>[4x]GMFASLIKRFQFVSVLDSNPQTKVMSLLGTIDNKDAIITAEKTHFLFDETVR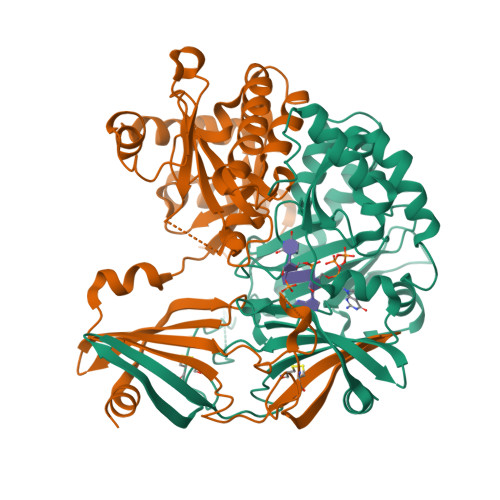RPSQDGRSTPVLYNCENEYSCINGIQELKEITSNDIYYWGLSVIKQDMESNPTAKLNLIWPATPIHIKKYEQQNFHLVRETPEMYKRIVQPYIEEMCNNGRLKWVNNILYEGAESERVVYKDFSEENKDDGFLILPDMKWDGMNLDSLYLVAIVYRTDIKTIRDLRYSDRQWLINLNNKIRSIVPGCYNYAVHPDELRILVHYQPSYYHFNIHIVNIKHPGLGNSIAAGKAILLEDIIEMLNYLGPEGYMNKTITYAIGENHDLWKRGLEEELTKQLERDGIPKIPKIVNGFK>[2x]ALYEDPPDQKTSPSGKPATLKICSWNVDGLRAWIKKKGLDWVKEEAPDILCLQETKCSENKLPAELQELPGLSHQYWSAPSDKEGYSGVGLLSRQAPLKVSYGIGDEEHDQEGRVIVAEFDSFVLVTAYVPNAGRGLVRLEYRQRWDEAFRKFLKGLASRKPLVLCGDL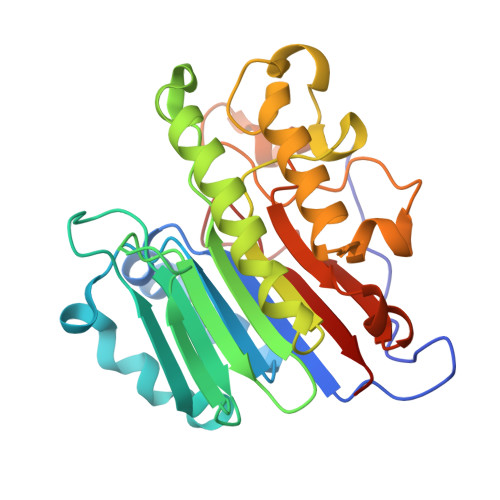NVAHEEIDLRNPKGNKKNAGFTPQERQGFGELLQAVPLADSFRHLYPNTPYAYTFWTYMMNARSKNVGWRLDYFLLSHSLLPALCDSKIRSKALGSDHCPITLYLAL(3S)-6'-chloro-5-(cyclobutylmethyl)-3',4,4',5-tetrahydro-2H,2'H-spiro[1,5-benzoxazepine-3,1'-naphthalene]-7-carboxylic 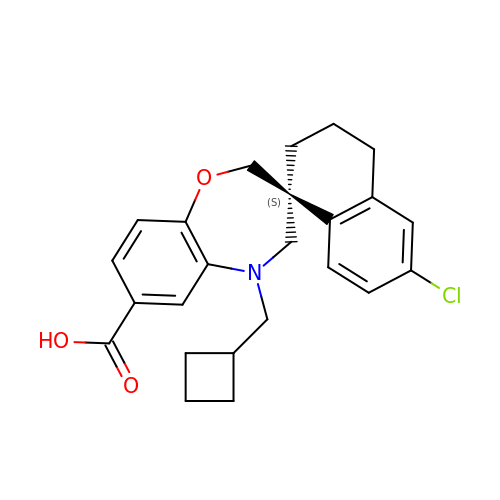acid | C24 H26 Cl N O3 | UZONKUOJBLOPMC-DEOSSOPVSA-N> 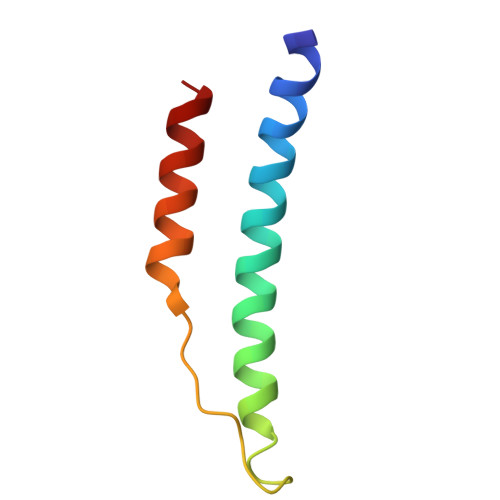KVQHIQLLQKNVRAQLVDMKRLEVDIDIKIRSCRGSCSRALAREVDLKDYEDQQKQLEQVIA>MKTIHVSVVTPDGPV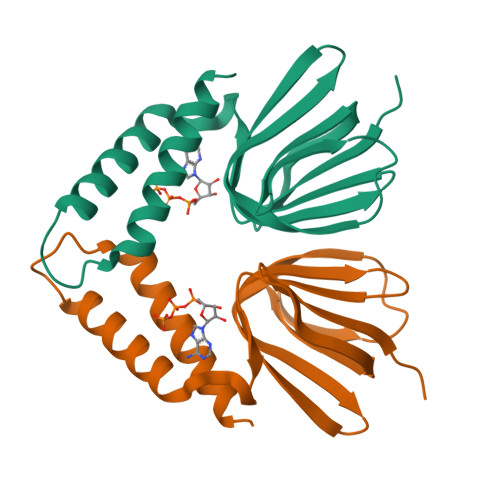YEDDVEMVSVKAKSGELGILPGHIPLVAPLEISAARLKKGGKTQYIAVSGGFLEVRPDKVTILAQAAERAEDIDVLRAKAAKERAERRLQSQQDDIDFKRAELALKRAMNRLSVAEMK[2x]AQPs are membrane-integral water channels that are present in all organisms where they facilitate passive flow of water across the membrane as a direct response to the osmotic pressure. Here, we present the first structural and functional characterization of a fish aquaporin; cpAQP1aa from the fresh water fish climbing perch (Anabas testudineus), a species that is of high osmoregulatory interest because of its ability to spend time in seawater and on land. These studies show that cpAQP1aa is a water-specific aquaporin with a unique fold on the extracellular side that results in a constriction region. The overall structure of cpAQP1aa shares most of the common AQP structural features; assembling as a homotetramer with each monomer forming a functional pore and consisting of six transmembrane α-helices (1–6) and five connecting loops (A-E).

To investigate if the conformation of loop C that is responsible for the cpAQP1aa extracellular constriction region is dependent on pH, we crystallized and solved the structure of cpAQP1aa at a lower pH; pH 6.5 instead of 7.8. The low pH crystals belonged to a different space group, C2221 instead of P4212, and diffracted to significantly lower resolution (3.5 Å). The lower diffraction quality is consistent with the differences in crystal packing; the crystals grown at the lower pH have considerably weaker crystal contacts and higher solvent content compared with the crystals at pH 7.8. Furthermore, in the structure at lower pH, there are four cpAQP1aa monomers in the asymmetric unit compared with one in the structure at higher pH. Because of this, structural differences can be observed between the monomers, most notably the fact that loops A and C could be built in their entirety in one of the monomers (monomer C). The two structures at different pH are very similar, although some minor differences can be seen in loops A and C. Nevertheless, the part of loop C that allows the formation of the extracellular constriction region (residues 114–119) occupies a similar position at both high and low pH. In particular, Tyr 107, Asn 116, Leu 117, Gly 118, and Arg 187 line up well and seem to be able to participate in the same hydrogen-bonding network in both structures (hydrogen bonds cannot be reliably assigned in the low pH structure because of the limited resolution). The channel profiles, as calculated by HOLE, are very similar in both structures, suggesting that the extracellular hydrophobic constriction region is unaffected by pH.

>[4x]MAREFKSKNFWKAVLAELVGMTLFIFLSLSAAIGNKNSTNPDQEVKVSLAFGLAIATLAQSLGHISGAHLNPAVTLGMLASCQISVLKAVMYIVAQMLGSALASGIVYGTRPNGNANLGLNALSGVTPSQGVGIELLATFQLVLCVIAVTDKRRRDVTGSAPLAIGLSVCLGHLAAISYTGCGINPARSFGPALILNNFENHWVYWVGPMCGGVAAALIYDFLLAPKFDDFPERIKVLVSGPVG>[4x]MQFRSIIRIVGLLLALFSVTMLAPALVALLYRDGAGVPFVTTFFVLLFCGAMCWFPNRRHKHELKSRDGFLIVVLFWTVLGSAGSLPFLIADNPNISVTDAFFESFSALTTTGATVIVGLDELPKAILFYRQFLQWFGGMGIIVLAVAILPVLGIGGMQLYRAEIPGPVKDTKMTPRIAETAKALWYIYLSLTIACAVAFWLAGMTPFDAISHSFSTIAIGGFSTHDASMGYFDSYAINLITVVFLLISACNFTLHFAAFASGGVHPKYYWKDPEFRAFIFIQVLLFLVCFLLLLKHHSYTSPYDAFDQALFQTVSISTTAGFTTTGFADWPLFLPVLLLFSSFIGGCAGSTGGGMKVIRILLLTLQGARELKRLVHPRAVYTIKVGGSALPQRVVDAVWGFFSAYALVFVVCMLGLIATGMDELSAFSAVAATLNNLGPGLGEVALHFGDVNDKAKWVLIVSMLFGRLEIFTLLILLTPTFWRS;>[4x]MKIIILGAGQVGGTLAENLVGENNDITIVDNNADRLRELQDKYDLRVVNGHASHPDVLHEAGAQDADMLVAVTNTDETNMAACQVAFTLFNTPNRVARIRSPEYLAEKEALFKSGAIPVDHLIAPEELVTSYIERLIQYPGALQVVSFAEQKVSLVAVKAYYGGPLVGNALSALREHMPHIDTRVAAIFRQGRPIRPQGTTIIEADDEVFFVAASNHIRSVMSELQRLEKPYRRIMIVGGGNIGASLAKRLEQTYSVKLIERDYQRAEKLSEQLENTIVFCGDAADQELLTEENIDQVDVFIALTNEDETNIMSAMLAKRMGAKKVMVLIQRGAYVDLVQGGVIDVAISPQQATISALLTHVRRADIVNVSSLRRGAAEAIEAVAHGDETTSKVVGRAIGDIKLPPGTTIGAVVRGEEVLIAHDRTVIEQDDHVVMFLVDKKYVPDVEALFQPSPFFL

TrkH, KtrB, and more distantly related KdpA belong to the superfamily of K+ transporters (SKTs) that are found in bacteria, fungi, and plants. TrkH or KtrB proteins assemble with their respective cytosolic partner proteins TrkA or KtrA to form a stable complex. To better understand the mechanism by which the Trk system functions, we determined the structures of TrkH-TrkA complex from V. parahaemalyticus in the presence of ADP (TrkHA-ADP), ATP (TrkHA-ATP), or ATPγS (TrkHA-ATPγS).

The TrkHA protein was crystallized in the presence of 10 mM ADP and the structure of TrkHA-ADP was solved by X-ray crystallography to a resolution of 3.53 Å (Rwork/Rfree = 0.25/0.29). TrkA forms a tetrameric ring, and each TrkA has a prominent non-protein density in the N2 domain in which we modeled as an ADP. Each TrkH protomer in the current TrkHA-ADP structure makes contact with the N1 and N2 domains of TrkA that we define as HN1 and HN2 interfaces. In the previous TrkHA-NADH structure, only the HN2 interface is resolved. TrkH remains a dimer and is in a closed conformation. In the TrkHA-ADP structure, each TrkH protomer makes contact with the TrkA ring in two places, the HN1 and HN2 interfaces. TrkH from the TrkHA-ADP is in a closed state, and the ion permeation pathway is constricted with a radius of 0.9 Å at the intramembrane loop immediately below the selectivity filter. ADP binds to the N2 domain and enables TrkA to form a tetrameric ring that holds TrkH shut by making contact with TrkH at both the HN1 and HN2 interfaces. These interactions, especially those at the HN1 interfaces, keep TrkH in a closed conformation. In the N2 domain, ATPγS and ADP interact with TrkA by an almost identical set of residues. ASP283 interacts with the adenosine ring, ASN306 and ASN24 interact with the α- and β-phosphate, respectively.> DLKYILETKLEEERNHLEELLEKVEEDYEG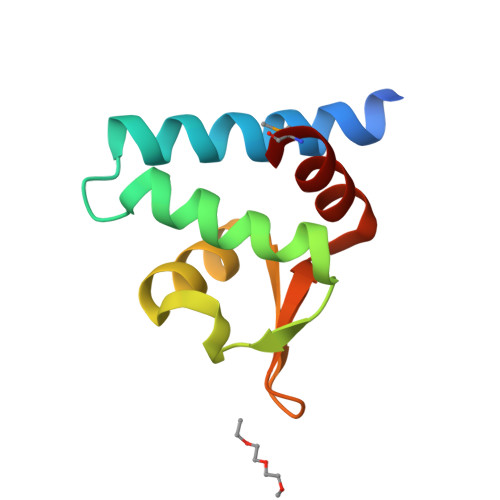INYDEVLEALKLFKDNYELPKSKIKRKIRIFLIKENILFLNPQKGTLKPQSYLVWNAIKRML>MLEKVETFDMNRVIDEFDEMTRNAHQVQKQTLKEILLKNQSAIYLQNCGLNGNATDPEEAFKSMVPLVTDVELEPYIKRMVDGDTSPILTGHPVPAISLSSGTSQGRPKFIPFTDELMENTLQLFRTAFAFRNRDFPIDDNGKALQFIFSSKQYISTGGVPVGTATTNVYRNPNFKAGMKSITSPSCSPDEVIFSPDVHQALYCHLLSGILFRDQVQYVFAVFAHGLVHAFRTFEQVWEEIVTDIKDGVLSNRITVPSVRTAMSKLLTPNPELAETIRTKCMSLSNWYGLIPALFPNAKYVYGIMTGSMEPYVPKLRHYAGDLPLVSHDYGSSEGWIAANVTPRLSPEEATFAVIPNLGYFEFLPVSETGEGEEKPVGLTQVKIGEEYEVVITNYAGLYRYRLGDVVKVIGFYNNTPQLKFICRRNLILSINIDKNTERDLQLSVESAAKRLSEEKIEVIDFSSYIDVSTDPGHYAIFWEISGETNEDVLQDCCNCLDRAFIDAGYVSSRKCKTIGALELRVVAKGTFRKIQEHFLGLGSSAGQFKMPRCVKPSNAKVLQILCENVVSSYFSTAF[2x];>HHHHHHMANLPILLDYWPSMFGMRARVALREKGVEFEYREEDFSNKSPLLLQSNPIHKKIPVLVHNGKPVCESL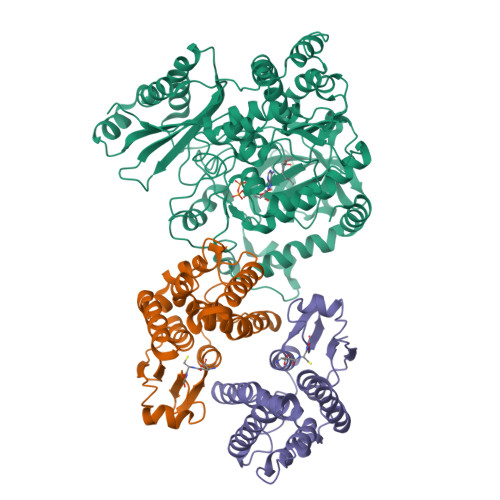NVVQYVDEAWPEKNPFFPSDPYGRAQARFWADFVDKKFTDAQFKVWGKKGEEQEAGKKEFIEAVKILESELGDKPYFGGDSFGYVDISLITFSSWFQAYEKFGNFSIESESPKLIAWAKRCMEKESVSKSLPDSEKIVAYAAEYRKNNL[4x]>[2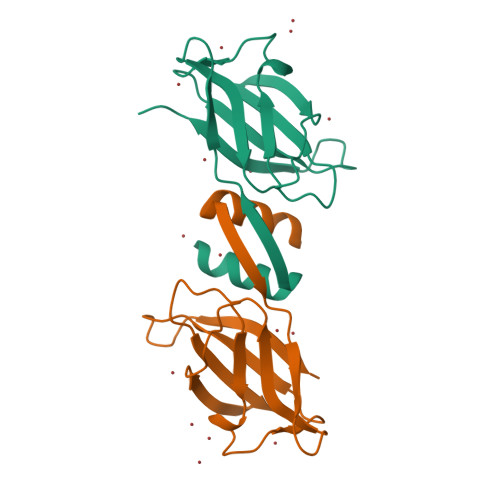x]XSATSLTFQLAYLVKKIDFDYTPNWGRGTPSSYIDNLTFPKVLTDKKYSYRVVVNGSDLGVESNFAVTPSGGQTINFLQYNKGYGVADTKTIQVFVVIPDTGNSEEYIIAEWKKT>GSHMKRFIGIRMRTITPSLVDELKASNPDFPEVSSGIYVQEVAPNSPSQRGGIQDGDIIVKVNGRPLVDSSELQEAVLTESPLLLEVR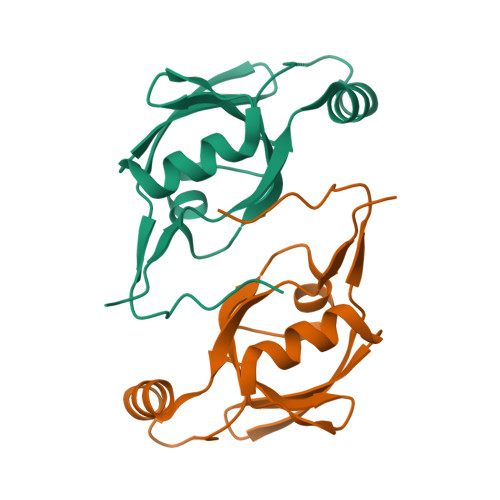RGNDDLLFSIAPEVVMGGGFGRWV[2x]> MRGSAHVVILGAGTGGMPAAYEMKEALGSGHEVTLISANDYFQFVPSNPWVGVGWKERDDIAFPIRHYVERKGIHFIAQSAEQIDAEAQNITLADGNTVHYDYLMIATGPKLAFENVPGSDPHEGPVQSIATVDHAERAFAEYQALLREPGPIVIGAMAGASCFGPAYEYAMIVASDLKKRGMRDKIPSFTFITSEPYIGHLGIQGVGDSKGILTKGLKEEGIE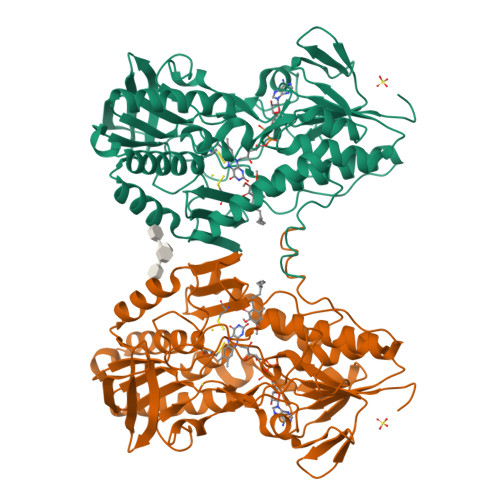AYTNCKVTKVEDNKMYVTQVDEKGETIKEMVLPVKFGMMIPAFKGVPAVAGVEGLCNPGGFVLVDEHQRSKKYANIFAAGIAIAIPPVETTPVPTGAPKTGYMIESMVSAAVHNIKADLEGRKGEQTMGTWNAVCFADMGDRGAAFIALPQLKPRKVDVFAYGRWVHLAKVAFEKYFIRKMKMGVSEPFYEKVLFKMMGITRLKEEDTHRKAS>[3x]RREQLMREEAEQK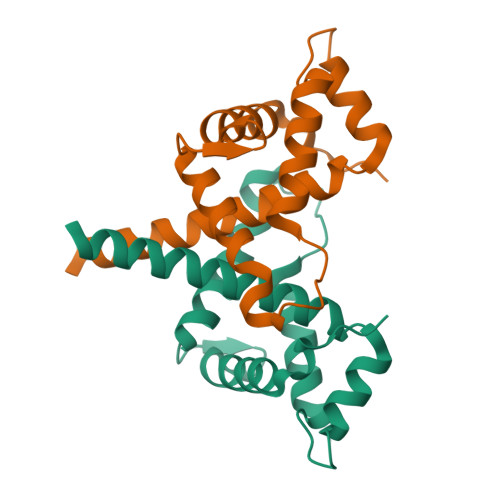RLKTVLELQYVLDKLGDDEVRTDLKQGLNGVPILSEEELSLLDEFYKLVDPERDMSLRLNEQYEHASIHLWDLLEGKEKPVCGTTYKVLKEIVERVFQSNYFDSTHN>[2x]EEIIWESLSVDVGSQGNPGIVEYKGVDTKTGEVLFEREPIPIGTNNMGEFLAI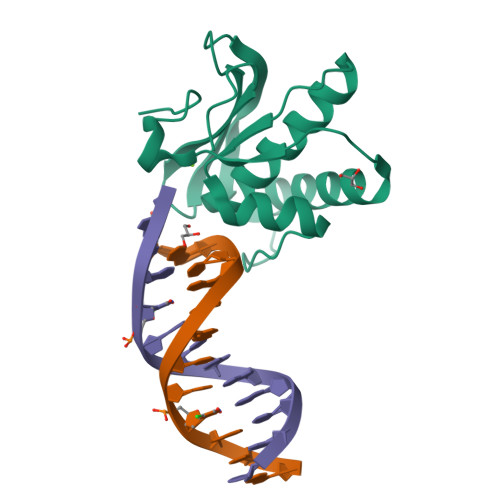VHGLRYLKERNSRKPIYSNSQTAIKWVKDKKAKSTLVRNEETALIWKLVDEAEEWLNTHTYETPILKWQTDKWGEIKADYG> SGHHEDSTDEASESSK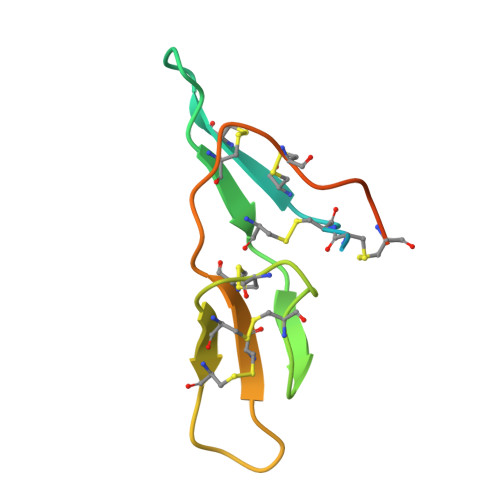PCCDRCECTKSIPPQCRCSDVRLNSCHSACKSCACTFSIPAQCFCGDINDFCYKPCKSSHSDDDDWN>MDILRKGNKDLIKDINRYTVLNLIREKGEITRTEIAKKCDFGMSTLTYILDDLQQEGIILEGAETSSTGGRRAKLVRFNKDYGFVVSVKVEEEQLLFALTDLNAEIIENTSIPFSSEKKPEEAIELIAKNVKKMCGNRDMNHLLGVGIAISGLVNRKKGTVIRSTMLGWENVALEAMLHAHFPDIPVYVDKNINCYTLAELWLGEGKQSNNFATVSVGAGLGLSVVINRQIYYGAQGGAGEFGHTTIQPGGYKCHCGQKGCLEMYASEFYFRNRGEELKEAYPTSELNDFHFDKVAKSARAGDEMATELMGKMGEYLGYGIRNIINTFNPEKVIIVGEGLHHRDLFLTKIDEIAS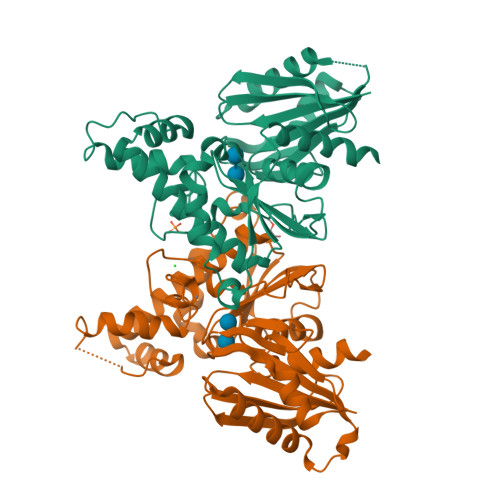QNFFSGAGFETEITTTSLEDPAWLQGAALLVIHQLFQVPIYEEEQTLLR[2x]> GSFLP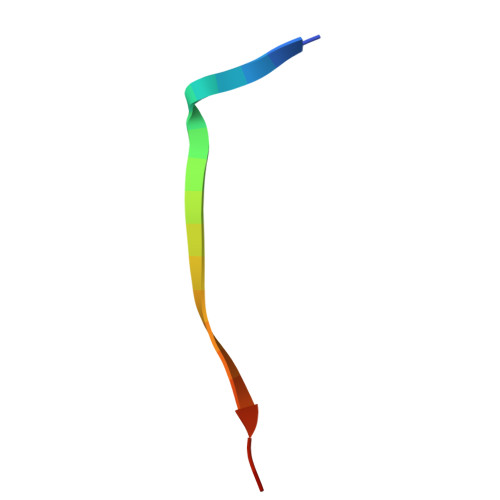NSEQQKSVDIVFSSP>[2x]GIDPFTMNAKPGFTDYIVKDIALADFGRKEISLAETEMPGLMATREEYGPKQPLKGARIAGSLHMTIQTAVLIETLAALGADIRWVSCNIYSTQDHAAAAIAAAGIPVFAVKGETLTEYWDYTAKLFDWHGGGTPNMILDDGGDATMLVHAGYRAEQGDTAFLDKPGSEEEEIFYALVKRLLKEKPKGWFAEIAKNIKGVSEETTTGVHRLYEMAN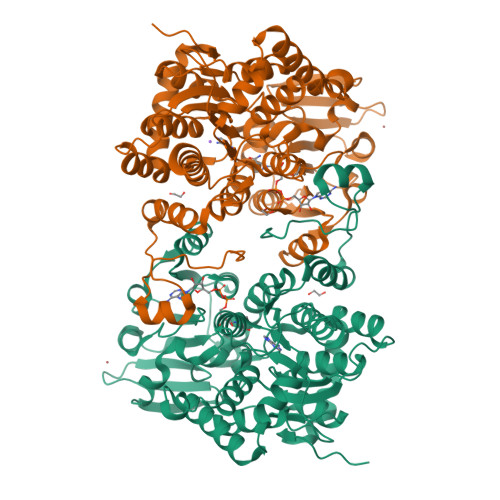KGTLLFPAINVNDSVTKSKFDNLYGCRESLVDGIRRGTDVMLSGKVAMVAGFGDVGKGSAASLRQAGCRVMVSEVDPICALQAAMEGYEVVTMEDAAPRADIFVTATGNKDIITIEHMRAMKDRAIVCNIGHFDNEIQIASLRNLKWTNIKPQVDEIEFPDKHRIIMLSEGRLVNLGNAMGHPSFVMSASFTNQTLAQIELFANNKDSKYAKKVYVLPKTLDEKVARLHLAKIGVKLTELRKDQADYIGVKQEGPYKSDHYRY> GGGGUGUGCCCGGCAUGGGUGCAGUCUAUAGGGUGAGAGUCCCGAACUGUGAAGGCAGAAGUAACAGUUAGCCUAACGCAAGGGUGUCCGUGGCGACAUGGAAUCUGAAGGAAGCGGACGGCAAACCUUCGGUCUGAGGAACACGAACUUCAUAUGAGGCUAGGUAUCAAUGGAUGAGUUUGCAUAACAAAACAAAGUCCUUUCUGCCAAAGUUGGUACAGAGUAAAUGAAGCAGAUUGAUGAAGGGAAAGACUGCAUUCUUACCCGGGGAGGUCU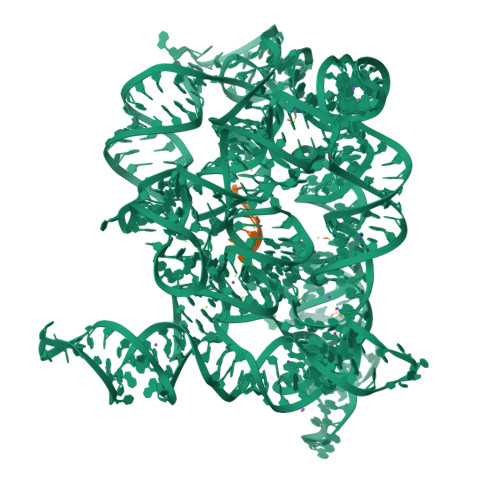GGAAACAGAAGUCAGCAGAAGUCAUAGUACCCUGUUCGCAGGGGAAGGACGGAACAAGUAUGGCGUUCGCGCCUAAGCUUGAACCGCCGUAUACCGAACGGUACGUACGGUGGUGUGG;> AUUUAUUA>MGSMYVVGHKIPDSDSICGAIALAYLKNQIGEPAIAARLGELSPETAFILEKFGFEAPEYKTSYAGEEVYIVDHSEITQAPDDIAQATIVGIVDHHKLGDLTTSTPLECWIRPVGCSNTVIKMMYDFYQVKIPANIAGIMMCAILSDTVIFKSPTCTTADIRCVEALAEIAGVEDFKEVGMDMFKVKSAVEGTPARDLVMRDFKDFNMNGNLVGIGQLEVIDL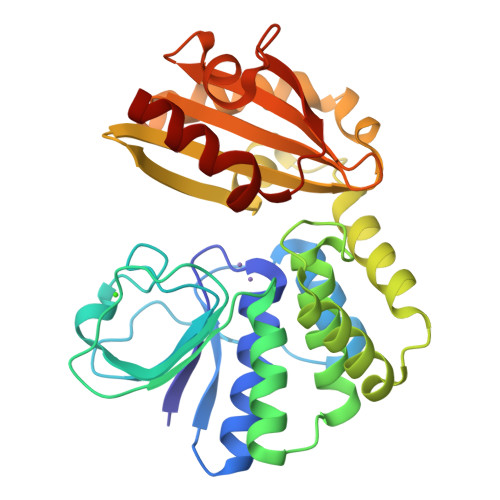AVFDDIKADLEADIAKLKVEGNRHSVLLLLTDIMKEGSEMLVVSDSADLTERAYGKPTVDGRVWLDGVLSRKKQVVPALQDAFQKV[4x]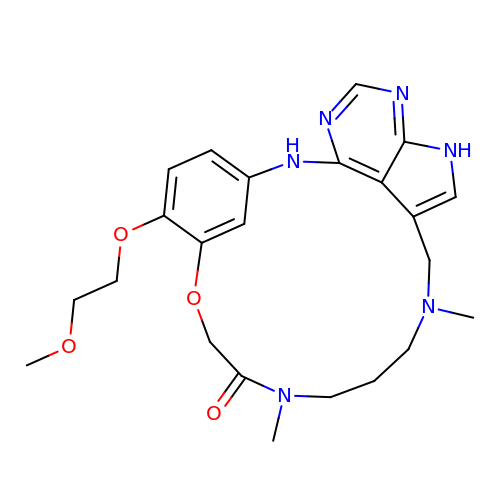6-(2-methoxyethoxy)-11,15-dimethyl-8-oxa-2,11,15,19,21,23-hexazatetracyclo[15.6.1.13,7.020,24]pentacosa-1(23),3(25),4,6,17,20(24),21-heptaen-10-one   | C23 H30 N6 O4 | HGGMHYCPDXPSRF-UHFFFAOYSA-N> GLECKPRPLHKTCSLFMRNIAPNISRAEIISLCKRYPGFMRVALSEPQPERRFFRRGWVTFDRSVNIKEICWNLQNIRLRECELSPGVNRDLTRRVRNINGITQHKQIVRNDIKLAAKLIHTLDDRTQLWASEPGTPPLPTSLPSQNPILKNITDYLIEEVSAEEEELLGSSGGAPPEEPPKEGNPAEINVERDEKLIKVLDKLLLYLRIVHSLDYYNTCEYPNEDEMPNRCGIIHVRGPMPPNRISHGEVLEWQKTFEEKLTPLLSVRESLSE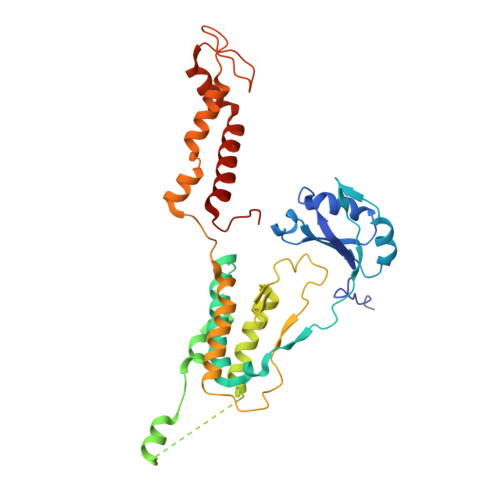EEAQKMGRKDPEQEVEKFVTSNTQELGKDKWLCPLSGKKFKGPEFVRKHIFNKHAEKIEEVKKEVAFFNNFLTDAKRPALPE> MGSDKIHHHHHHENLYFQGMLNFTVGPVMSSEEVRAIGAEQVPYFRTTEFSSTMLENEKFMLEYAKAPEGSKAVFMTCSSTGSMEAVVMNCFTKKDKVLVIDGGSFGHRFVQLCEIHEIPYVALKLEHGKKLTKEKLYEYDNQNFTGLLVNVDETSTAVLYDTMMIGEFCKKNNMFFVCDCV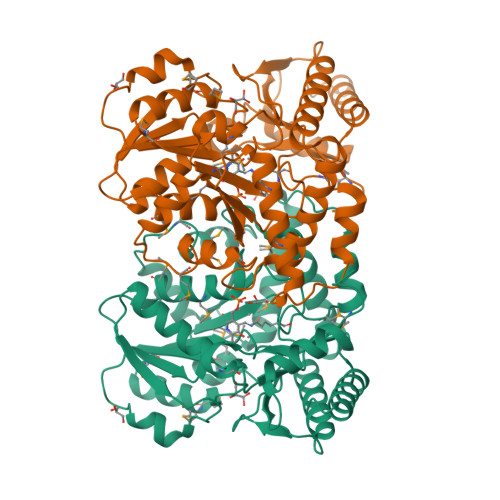SAFLADPFNMNECGADVMITGSQKVLACPPGISVIVLAPRGVERVEKSKVRTMYFDLKDALKNQERGQTPFTPAVGILLQINERLKEIKKHGGADAEVARIASQAADFRAKIKDLPFELVSESPANGVTSVHPTTANAYDIFLKLKDEYGIWICPNGGEMKDTIFRVGHIGALTHEDNTTLVNAFKDLQKRNLL> SMADLLVPKLTASVTDGAVGVTVDAPVSVTAADGVLAAVTMVNDNGRPVAGRLSPDGLRWSTTEQLGYNRRYT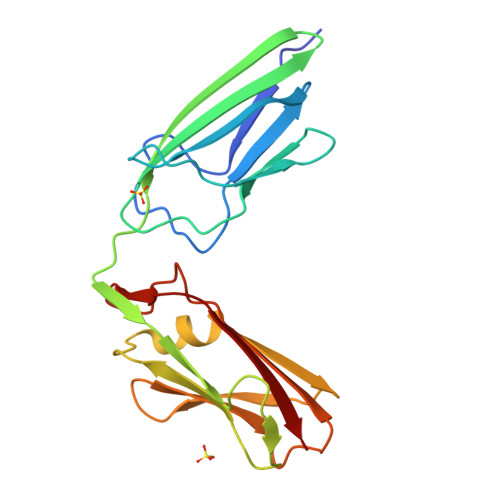LNATALGLGGAATRQLTFQTSSPAHLTMPYVMPGDGEVVGVGEPVAIRFDENIADRGAAEKAIKITTNPPVEGAFYWLNNREVRWRPEHFWKPGTAVDVAVNTYGVDLGEGMFGEDNVQTHFTIG pyridine | C5 H5 N | 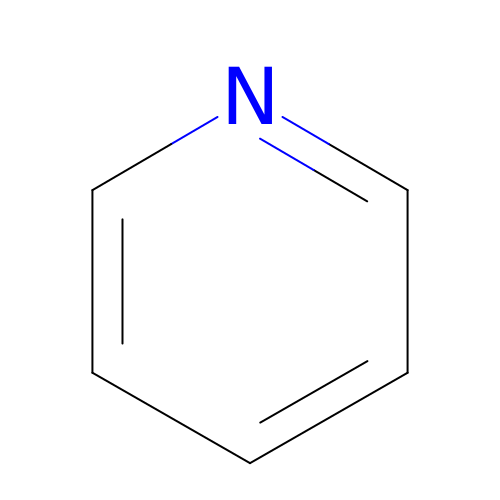JUJWROOIHBZHMG-UHFFFAOYSA-N>MPMTVITLKNVPQSLRGDLTRWMQEIATGVYVGNFNSRIREYLWRRVQETMGAGEASMCFAARNELGYDFLTENASRSVIDYDGLPLIFIPKE[2x];>[4x]MAGPIIAGKSESSELPRVEDRATFIYIEHAKINRVDS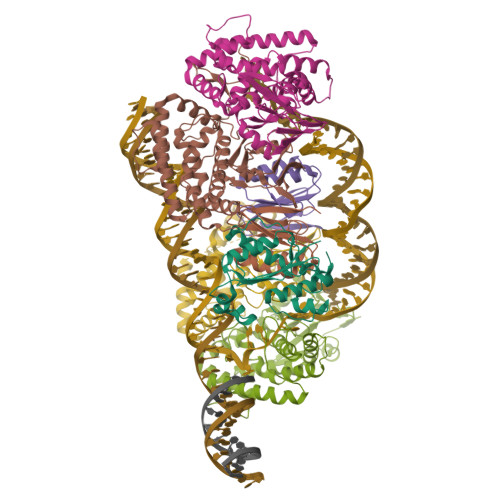AVTVAEAKGVVRIPAAMIGVLLLGPGTDISHRAVELLGDTGTALVWVGEQGVRYYASGRALARSTRFLVKQAELVTNERSRLRVARRMYQMRFPTEDVSKLTMQQLRSHEGARVRRKYRELSKKYNVPWKKRVYNPDDFAGGDPINQALSAAHVALYGLVHSVVAALGLSPGLGFVHTGHDRSFIYDVADLYKAEITVPIAFAVAAEAEEGQDIGQLARLRTRDAFVDGKILKRMVKDLQTLLEIPEEGQIEAEPLSLWDDKEKLVPYGVNYSE;> IRYVVIDIETDGKDAKRNHILEIGAIRCEDGKETHFTALISGDAVPPSITKLTGITATLLQKEGQEEKKVLTAFREFIGDDDLVGYHVSFDIEFLRQAFKKYGLGYLKNKTHDLLRIVKKEQLFQADYKLETSLQSYGIHKKVPHRALGDAELVKCLAKKLNKF1-deoxy-5-O-phosphono-1-(3,3,4,5-tetramethyl-9,11-dioxo-2,3,8,9,10,11-hexahydro-7H-quinolino[1,8-fg]pteridin-12-ium-7-yl)-D-ribitol | C22 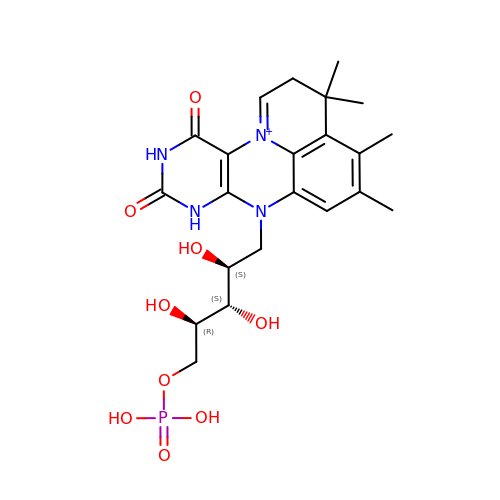H30 N4 O9 P | KOUJZPGFPGLHCZ-IYOUNJFTSA-O>MSCPVTTEGDYVWKISEFYGRKPEGTYYNSLGFNIKATNGGTLDFTCSAQADKMEDHKWYSCGENSFMNFSFGSDRSGLLLKQKVSDDITYVATATLPNYCRAGGNGPKDFVCQGVADAYITLVTLPKSS[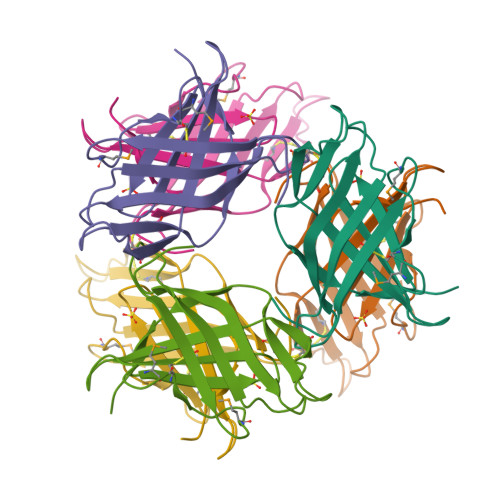2x]>[2x]MGSSHHHHHHSSGLVPRGSHMASGLYPSYNTSPAAPDSTGMQSTAVQLAGKIRLGWNIGNTMEAIGGETAWGNPMVSNELLKLVKDSGFDAVRIPVAWDQYANQESAEISAAWLNRVKQVVQMAIDNELYVLINIHWDGGWLE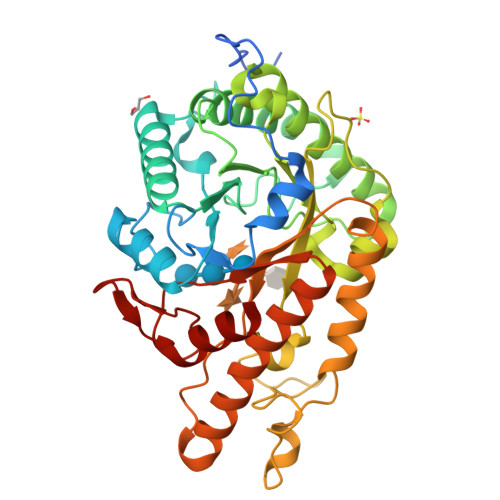NNITPAKKDENNAKQKAFWEQIATHLRDFDEHLLFAGTNAPNAENAEQMDVLNSYLQTFVDAVRSTGGKNAYRVLVLQGPVTDIEKTNELWTHMPADTATDRLMAEVHFYTPYNFALMRQDESWGKQFYYWGEGFLSTTDTERNPTWGEEATIDQLFDLMKTKFVDQGIPVVLGEFSAMRRTNLTGDALTLHLAGRAYYHKYVTQQALARGLLPFYWDNGGNDNFSSGIFNRQQNTVFDQQVLDALLEGAGAQ> MTRLFMLVCLGIVCQGTTGNILRGESLNKSLPILHEWKFFDYDFGSDERRQDAILSGEYDYKNNYPSDIDQWHDKIFVTMLRYNGVPSSLNVISKKVGDGGPLLQPYPDWSFAKYDDCSGIVSASKLAIDKCDRLWVLDSGLVNNTQPMCSPKLLTFDLTTSQLLKQVEIPHDVAVNATTGKGRLSSLAVQSLDCNTNSDTMVYIADEKGEGLIVYHNSDDSFHRLTSNTF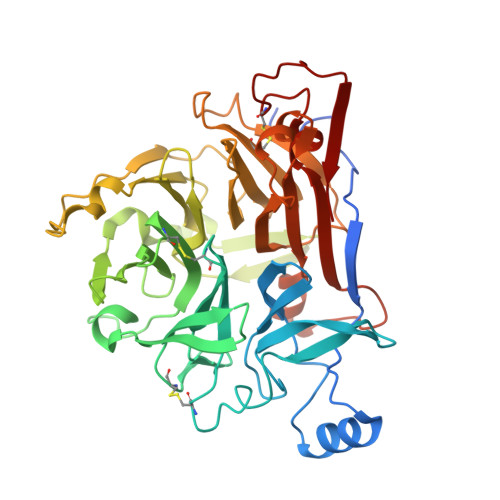DYDPKFTKMTIDGESYTAQDGISGMALSPMTNNLYYSPVASTSLYYVNTEQFRTSDYQQNDIHYEGVQNILDTQSSAKVVSKSGVLFFGLVGDSALGCWNEHRTLERHNIRTVAQSDETLQMIASMKIKEALPHVPIFDRYINREYILVLSNKMQKMVNNDFNFDDVNFRIMNANVNELILNTRCENPDNDRTPFKISIHL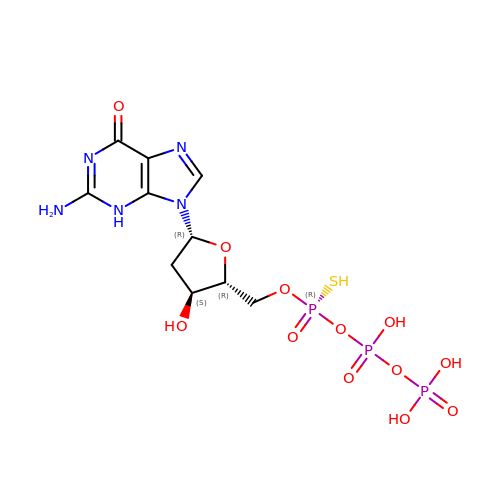2'-deoxyguanosine-5'-O-(1-thiotriphosphate) | C10 H16 N5 O12 P3 S | IOCRYHATDKHWPM-KUFCIHQDSA-N>[8x]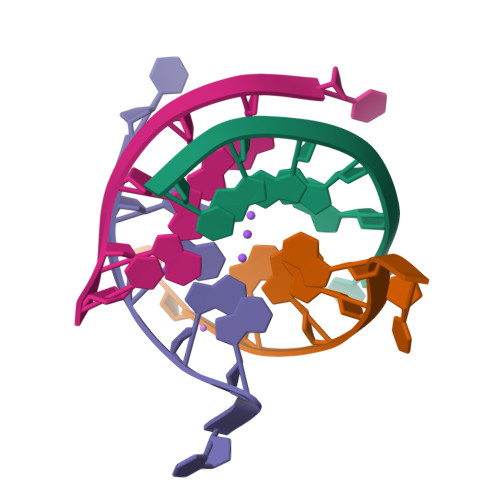TGGGGT> SNAMFAPQGLAQFIKVNVTLENGEPVFIFTDANGQVCQGDITVTQAGTI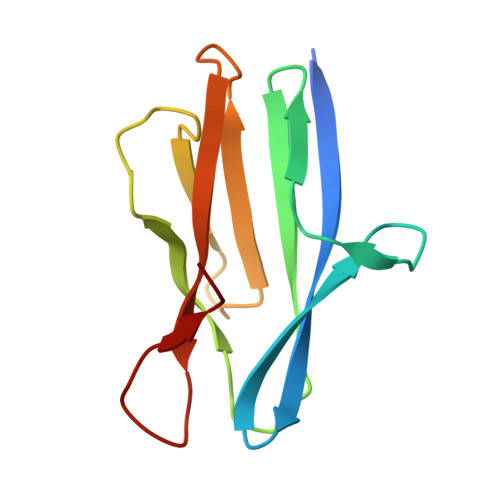TYLLNDQTLKGLKFVGVGFVTPFDGIIDAVTISSDGMLVQLVDLDKTPGTTKFQFVLSNTANTLLVLSPD>GSHMGLKIRQRQRFGRLELKRISGRGFKNDEEILIGNGTIQKIGIWDGEEEFHVRCGECRGILKKSKMKLEKLLINSAKKEDMRDLIILCMVFSQDTRMFQGVRGEINFLNRAGQLLSPMYQLQRYFLNRSSDLFDQW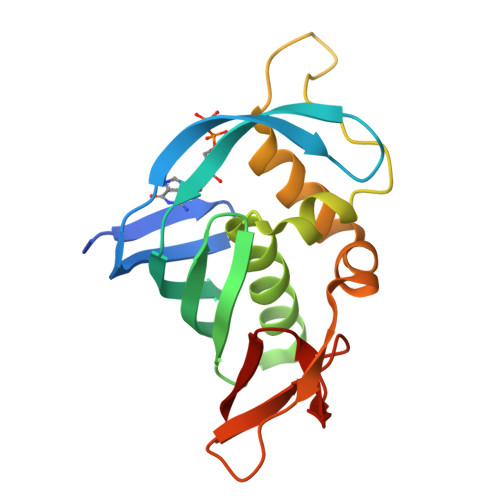GYEESPKASELHGINESMNASDYTLKGVVVTKN[2x]>GPMSPLLHSLVGQHILSVQQFTKDQMSHLFNVAHTLRMMVQKERS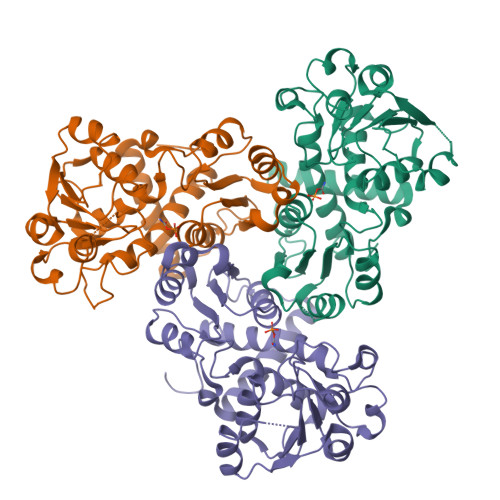LDILKGKVMASMFYEVSTRTSSSFAAAMARLGGAVLSFSEATSSVQKGESLADSVQTMSCYADVVVLRHPQPGAVELAAKHCRRPVINAGDGVGEHPTQALLDIFTIREELGTVNGMTITMVGDLKHGRTVHSLACLLTQYRVSLRYVAPPSLRMPPTVRAFVASRGTKQEEFESIEEALPDTDVLYMTRIQKERFGSTQEYEACFGQFILTPHIMTRAKKKMVVMHPMPRVNEISVEVDSDPRAAYFRQAENGMYIRMALLATVLGRF[6x]> SANNPWTGFQIFLSPYYAN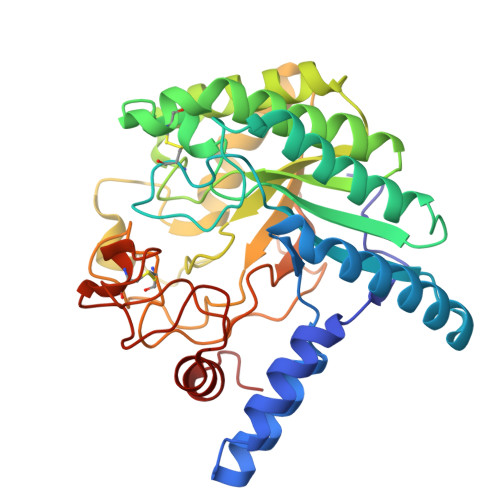EVAAAAKQITDPTLSSKAASVANIPTFTWLDSVAKIPDLGTYLASASALGKSTGTKQLVQIVIYDLPDRDCAAKASNGEFSIANNGQANYENYIDQIVAQIQQFPDVRVVAVIEPDSLANLVTNLNVQKCANAKTTYLASVNYALTNLAKVGVYMYMDAGHAGWLGWPANLSPAAQLFTQVWQNAGKSPFIKGLATNVANYNALQAASPDPITQGNPNYDEIHYINALAPLLQQAGWDATFIVDQGRSGVQNIRQQWGDWCNIKGAGFGTRPTTNTGSQFIDSIVWVKPGGECDGTSNSSSPRYDSTCSLPDAAQPAPEAGTWFQAYFQTLVSAANPPL>ERGEVYSEKMFTESERTYFMNVKENRKGDYFLNIVESKRSPSGDFERHSIFVYEENMNEFESNLLKAIAVIKQKVSTGSVGSSAR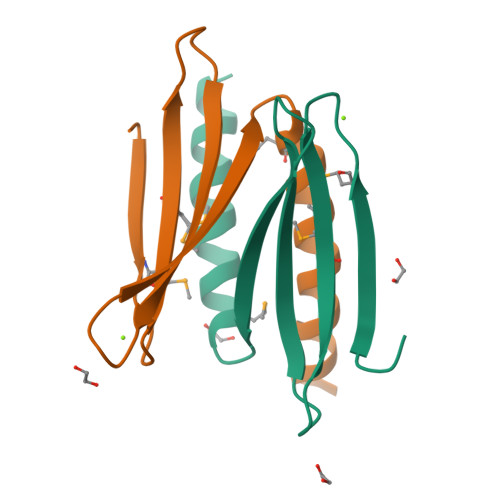HNKGYGEYGERSK[2x]>[6x]KSKSDVFHLGLTKNDLQGAQLAIVPGDPERVEKIA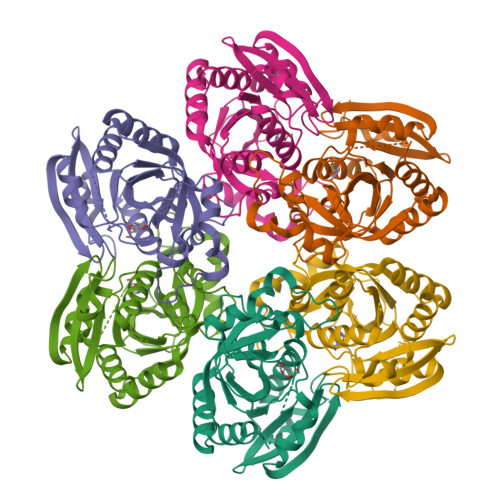ALMDKPVKLASHREFTSWRAELDGKAVIVCSTGIGGPSTSIAVEELAQLGIRTFLRIGTTGAIQPHINVGDVLVTTASVRLDGASLHFAPMEFPAVADFACTTALVEAAKSIGATTHVGVTASSDTFYPGQERYDTYSGRVVRRFKGSMEEWQAMGVMNYEMESATLLTMCASQGLRAGMVAGVIVNRTQQEIPNAETMKQTESHAVKIVVEAARRLL>MKHLTEEQKLTLDMVRDVATREIAP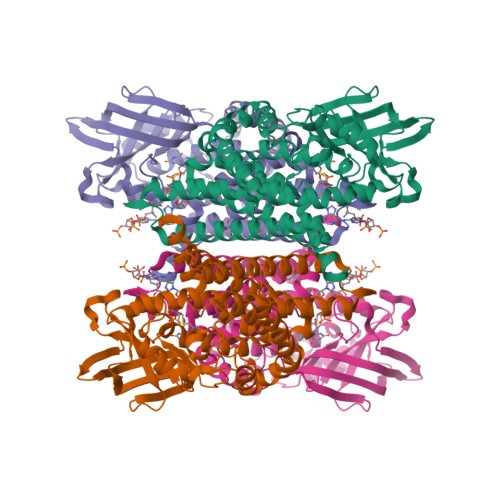RALELDEKSLFPEYARDLFAKLGLLNPLLPAAYGGTEMGVLTLALILEELGRVCASTALLLIAQTDGMLPIIHGGSPELKERYLRRFAGESTLLTALAATEPAAGSDLLAMKTRAVRQGDKYVINGQKCFITNGSVADVIVVYAYTDPEKGSKGISAFVVEKGTPGLVYGRNESKMGMRGSINSELFFENMEVPAENIIGAEGTGFANLMQTLSTNRVFCAAQAVGIAQGALDIAVRHTQDRVQFGKPIAHLAPVQFMVADMATAVEASRLLTRKAAELLDDGDKKAVLYGSMAKTMASDTAMRVTTDAVQVLGGSGYMKENGVERMMRDAKLTQIYTGTNQITRMVTGRALLFPKGELNSKLEGKPIPNPLLGLDSTRTGHHHHHH[4x]>[2x]MTQFNPVDHPHRRYNPLTGQWILVSPHRAKRPWEGAQETPAKQVLPAHDPDCFLCAGNVRVTGDKNPDYTGTYVFTNDFAALMSDTPDAPESHDPLMRCQSARGTSRVICFSPDHSKTLPELSVAALTEIVKTWQEQTAELGKTYPWVQVFEN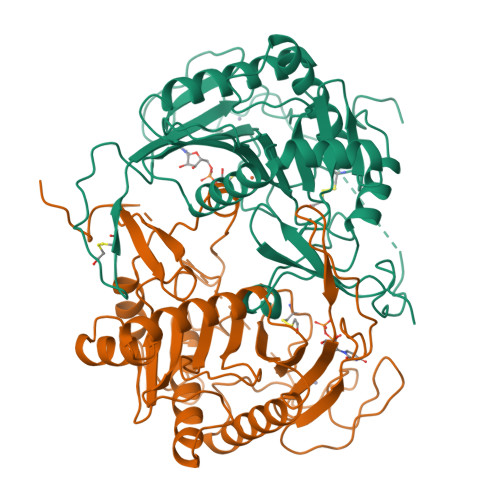KGAAMGCSNPHPHGQIWANSFLPNEAEREDRLQKEYFAEQKSPMLVDYVQRELADGSRTVVETEHWLAVVPYWAAWPFETLLLPKAHVLRITDLTDAQRSDLALALKKLTSRYDNLFQCSFPYSMGWHGAPFNGEENQHWQLHAHFYPPLLRSATVRKFMVGYEMLAETQRDLTAEQAAERLRAVSDIHFRESGV>[4x]MVARPKSEDKKQALLEAATQAIAQSGIAASTAVIARNAGVAEGTLFRYFATKDELINTLYLHLKQDLCQSMIMELDRSITDAKMMTRFIWNSY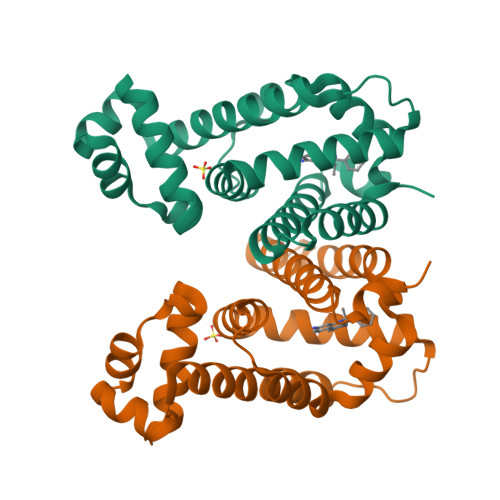ISWGLNHPARHRAIRQLAVSEKLTKETEQRADDMFPELRDLCHRSVLMVFMSDEYRAFGDGLFLALAETTMDFAARDPARAGEYIALGFEAMWRALTREEQ>[2x]TPNKEDYLKCLYELGTRHNKITNKEIAQLMQVSPPAVTEMMKKLLAEELLIKDKKAGYLLTDLGLKLVSDLYRKHRLIEVFLVHHLGYTTEEIHEEAEVLEHTVSDHFVERL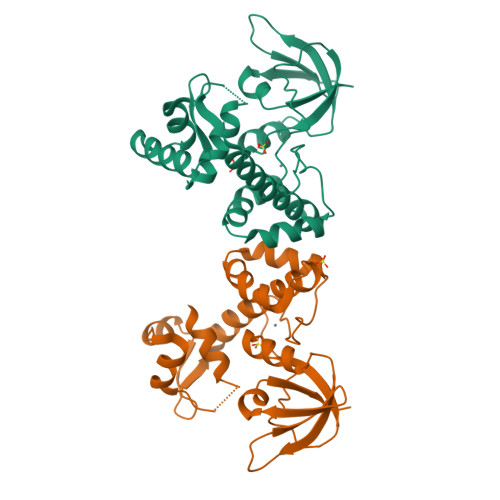DQLLDYPKACPHGGTIPAKGELLVEKHKLTLEEAKEKGDYILARVHDNFDLLTYLERNGLQVGKTIRFLGYDDFSHLYSLEVDGQEIQLAQPIAQQIYVEKI> MSSLSRELVFLILQFLDEEKFKETVHKLEQESGFFFNMKYFEEKVHAGEWDEVEKYLSGFTKVDDNRYSMKIFFEIRKQKYLEALDRHDRAKAVDILVKDLKVFSTFNEELYKEITQLLTLENF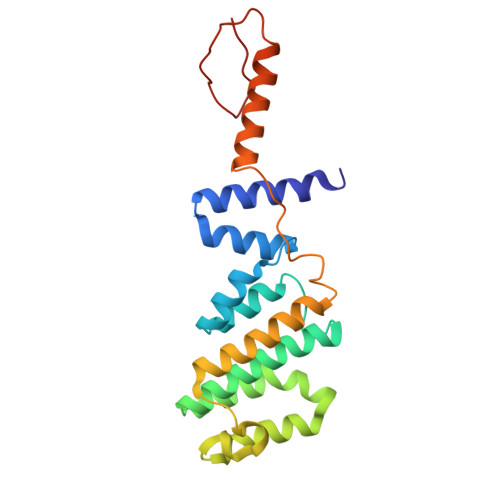RENEQLSKYGDTKSARSIMLIELKKLIEANPLFREKLVFPTLKASRLRTLINQSLNWQHQLCKNPRPNPDIKTLFTDHTCTPPNG> EIQMPTHKDLNLDITIELPDREVPIRYRINYENALLARTVETKLNQDITVTASGDGKATMTILTFYNAQLQEKANVCNKFHLNVSVENIHLNAMGAKGALMLKICTRYLGEVDSTMTIIDISMLTGFLPDAEDLTRLSKGVD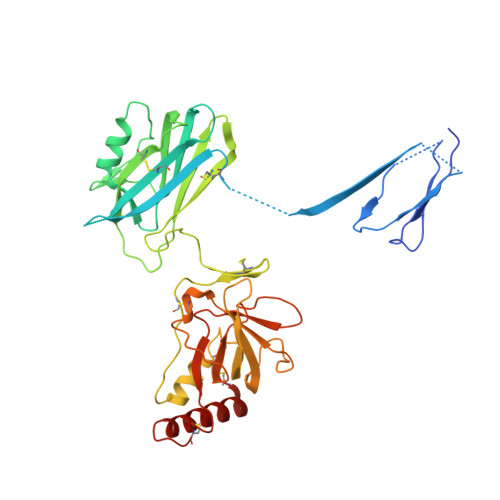RYISRYEVDNNMAQKVAVIIYLNKVSHSEDECLHFKILKHFEVGFIQPGSVKVYSYYNLDEKCTKFYHPDKGTGLLNKICIGNVCRCAGETCSSLNHQERIDVPLQIEKACETNVDYVYKTKLLRIEEQDGNDIYVMDVLEVIKQGTDENPRAKTHQYISQRKCQEALNLKVNDDYLIWGSRSDLLPTKDKISYIITKNTWIERWPHEDECQEEEFQKLCDDFAQFSYTLTEFGCPT> MRVALTIAGSDSGGGAGVQADLKVFFRFGVYGTSALTLVTAQNTLGV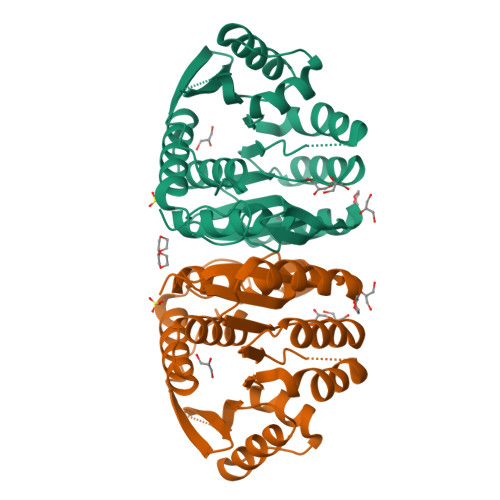QRVHLLPPEVVYAQIESVAQDFPLHAAKTGALGDAAIVEAVAEAVRRFGVRPLVVDPVMVAKSGDPLLAKEAAAALKERLFPLADLVTPNRLEAEALLGRPIRTLKEAEEAAKALLALGPKAVLLKGGHLEGEEAVDLLATRGGVLRFSAPRVHTRNTHGTGCTLSAAIAALLAKGRPLAEAVAEAKAYLTRALKTAPSLGHGHGPLDHWA> GPDSMVLLSSSWLPLNKDIEVEVVDYLPSSSVAPDLFALTLLRINDSSMKEKYDSMHEKMNAYAQIVPFDSELEIGYDGVFRDAPRSVRRVRRISATKLYLVDFGKIINYEKAKCFQLPKVFQSMPTRVSLCGLDGLTWSPV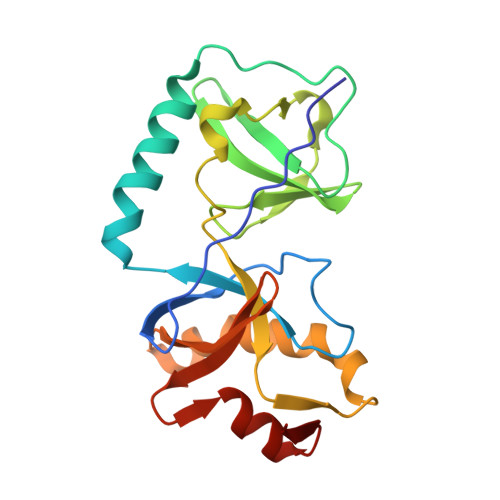AIPSFDNIREVVKKWGQMENSTLHAMACGFQGSINMINLFCGKSILADRLQRKGVCEYL> GACLSIPNFPVHITGKTQQLHVGPKPSIARFSFNPFDLGTVFNRFQSLCAHLEGYSGDLIVNWLVTCSALTNARLYIIPVYDNYSFEKFSEEKLIQCKYEFKQISLVRKGTVHIPFVNWFGSYSRTRFPKLLFYFPNGVSGPSGEKIHVTVQLDRILNFSGLGHRLFKEIGPLVGE;> GSDPFSFLLNYSHCGTLVESSLNKGGMWCVPVSPVNLAAYTLQGEALVFNDAFVSKTHNWLHFMASTTAYWRGTLHYQMRVTYKDRNAACRNLVAFYTTNNESLFGFNNKPVGDTGISSVMGDSFSVDITVPFLIPTCYLQTIRGKFDYLNSCNGCIYFHLPTKSATSVQLWVRPGQDFDFARFRLLKAGYT;> GPDFTKIIWPTVVERNFSNPQSEITTTLQELYGDTFETVSICPPQSYGGELLKGKIFFSSTPEFTREDLVEGKILASFKLDEVLSGLGMGAMLMTQIMSGHATIRVSAKVMLSKFCSFALKLVYDELMQLNSDTTDFGKISVLPGAIFSTQEEEFSFDFELFSPGVHLK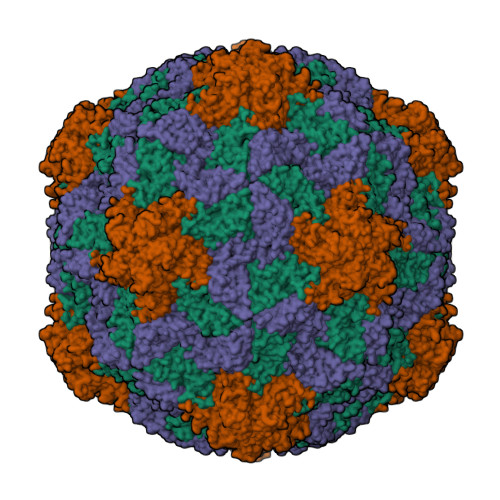FDNNKLLGKVHLAALSAPNLTENMPESFSCTFNFSIVDVKTTFYNIGQ> GPAMLTTRIIKETEKLQKECPPGITATPTKENPRYFMVTIQGPPQSCYEGGLFRLELFLPEEYPMKPPKVRFLTRIYHPNVDKVGRICLDIIKDKWSPALLINKVLLSIQILMSSP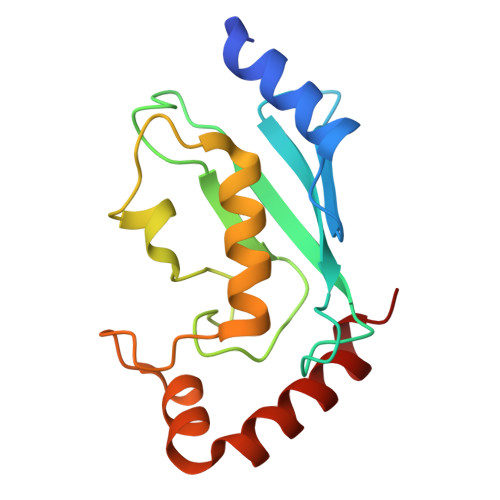NPDDPLANDVAEHWKEDEASALQTAREWTRKYAKP> GAMGSMPHRTIHLFRKGLRLHDNPTLLAALESSETIYPVYVLDRRFLASAMHIGALRWHF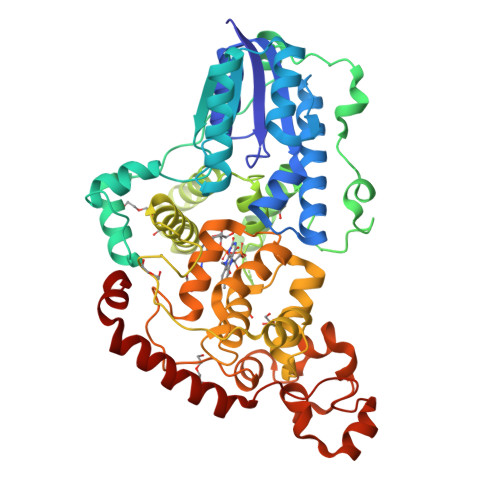LLQSLEDLHKNLSRLGARLLVIQGEYESVLRDHVQKWNITQVTLDAEMEPFYKEMEANIRRLGAELGFEVLSRVGHSLYDTKRILDLNGGSPPLTYKRFLHILSQLGDPEVPVRNLTAEDFQRCMSPEPGLAERYRVPVPADLEIPPQSLSPWTGGETEGLRRLEQHLTDQGWVANFTKPRTIPNSLLPSTTGLSPYFSMGCLSVRTFFQRLSNIYAQAKHHSLPPVSLQGQLLWREFFYTVASATQNFTQMAGNPICLQIHWYEDAERLHKWKTAQTGFPWIDAIMTQLRQEGWIHHLARHAVACFLTRGDLWISWEEGMKVFEELLLDADYSINAGNWMWLSASAFFHHYTRIFCPVRFGKRTDPEGQYIRKYLPVLKNFPTKYIYEPWTASEEEQRQAGCIIGRDYPFPMVNHKEASDRNLQLMRRVREEQRGTAQLTR The core enzyme in the replication machinery is the viral RNA-dependent RNA polymerase (RdRP) 3Dpol. The enzyme adopts the canonical closed right-hand polymerase fold, consisting of fingers, palm, and thumb subdomains that encircles seven conserved structural motifs (A to G), playing critical roles in rNTP substrate recognition, template/primer binding and catalysis. 3Dpol uses 3B as a primer protein to initiate the replication process. Unlike other picornaviruses, the animal pathogen foot-and-mouth disease virus (FMDV), encodes three non-identical copies of the 3B (3B1, 3B2, and 3B3) that could be specialized in different functions within the replication complex.

Different crystals were of complexes: 3DpolHis-3B1, 3DpolHis-3B3 or 3DpolStop-3B1, 3DpolStop-3B3 that belonged to the space group P3221. While in orthorhombic crystals the bound 3B1 peptide connected the two 3Dpol molecules of the asymmetric unit, in the P3221 space group, the proximity of a neighbour 3Dpol molecule in the crystal packing prevented the correct binding of the whole 3B peptide, and only a few residues could be positioned in the electron density maps. In these crystals, the position of the visible 3B1 fragment is almost coincident with that of 3B3 (from G5 to P10), therefore, the final structural analysis was carried out only with the 3DpolStop-3B3 complex structure that diffracted at the highest resolution (1.85 Å). As expected, the visible part of the FMDV 3B3 peptide in the trigonal crystals bound to the same 3Dpol cavity at the base palm, close to residues from Y323 to V326 and from Y346 to L348. This binding cavity was also equivalent to the so-called “contact II region” in enterovirus 71 (EV71) 3Dpol, involving residues: from T313 to I317 and from Y335 to P338 that anchor the second half of the EV71 3B peptide, amino acids from L11 to R17. The proximity of a neighbouring 3Dpol molecule (Grey) in the crystal packing probably limits the 3B molecule from being arranged in an ordered way. Also, L19 is replaced by N in 3B3, hindering the placement of this residue in the hydrophobic pocket. In light of these data we suggest that 3B2 and 3B3 could bind 3Dpol through region I which has a lower affinity.

> GLIVDTRDVEERVHVMRKTKLAPTVAHGVFNPEFGPAALSNKDPRLNEGVVLDEVIFSKHKGDTKMSAEDKALFRRCAADYASRLHSVLGTANAPLSIYEAIKGVDGLDAMEPDTAPGLPWALQGKRRGALIDFENGTVGPEVEAALKLMEKREYKFACQTFLKDEIRPMEKVRAGKTRIVDVLPVEHILYTRMMIGRFCAQMHSNNGPQIGSAVGCNPDVDWQRFGTHFAQYRNVWDVDYSAFDANHCSDAMNIMFEEVFRTEFGFHPNAEWILKTLVNTEHAYENKRITVEGGMPSGCSATSIINTILNNIYVLYALRRHYEGVELDTYTMISYGDDIVVASDYDLDFEALKPHFKSLGQTITPADKSDKGFVLGHSITDVTFLKRHFHMDYGTGFYKPVMASKTLEAILSFARRGTIQEKLISVAGLAVHSGPDEYRRLFEPFQGLFEIPSYRSLYLRWVNAVCGDAAALEHHHHHH;> GPYEGPVKKPVALKVKAKNLIVTE> MALPLLASRRLFSSFVFRGQPSTLSSNLSLVRIRGLHGGSLSPPSATLPRAVQLFS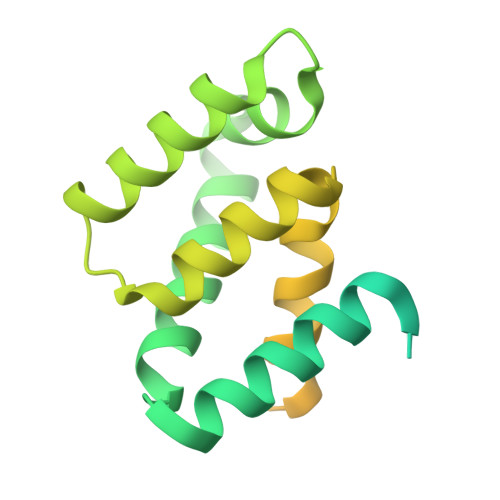SRIAFSTAAAEDSGASQTLEGRYASALFRVAKKKNQLEKVYGDLESVRNALKDSSEFRLFVDSPAVSVQQKLDVLRQLVNRYKFDPLTGNLLTTLVENKRLPMLARVADAFDAMYRKEKGEVKCLVTSAKPLSAQQQKEIVAALQNRAGTQARLIIDYAVSPQIMGGLVVRLGEQVLDFSVATRLDRLQSQLLAPL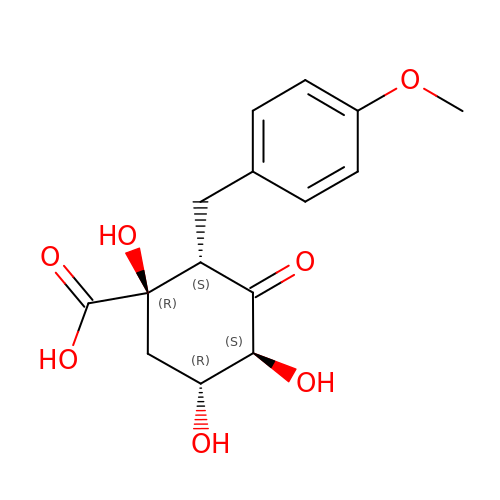(1R,2S,4S,5R)-2-(4-methoxyphenyl)methyl-1,4,5-trihydroxy-3-oxocyclohexane-1-carboxylic acid | C15 H18 O7 | KDOXKRDIRCHNDT-UQFNBPPOSA-N> SELLVNTKSGKVMGTRVPVLSSHISAFLGIPFAEPPVGNMRFRRPEPKKPWSGVWNASTYPNNCQQYVDEQFPGFSGSEMWNPNREMSEDCLYLNIWVPSPRPKSTTVMVWIYGGGFYSGSSTLDVYNGKYLAYTEEVVLVSLSYRVGAFGFLALHGSQEAPGNVGLLDQRMALQWVHDNIQFFGGDPKTVTIFGESAGGASVGMHILSPGSRDLFRRAILQSGSPNCPWASVSVAEGRRRAVELGRNLNCNLNSDEELIHCLREKKPQELIDVEWNVLPFDSIFRFSFVPVIDGEFFPTSLESMLNSGNFKKTQILLGVNKDEGSFFLLYGAPGFS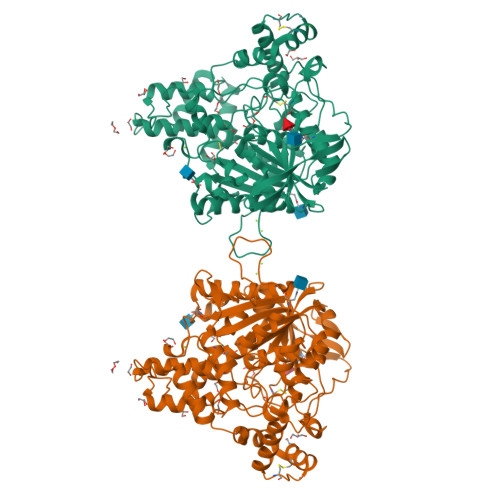KDSESKISREDFMSGVKLSVPHANDLGLDAVTLQYTDWMDDNNGIKNRDGLDDIVGDHNVICPLMHFVNKYTKFGNGTYLYFFNHRASNLVWPEWMGVIHGYEIEFVFGLPLVKELNYTAEEEALSRRIMHYWATFAKTGNPNEPHSQESKWPLFTTKEQKFIDLNTEPMKVHQRLRVQMCVFWNQFLPKLLNAT> MAKMAFTLADRVTEEMLADKAALVVEVVEENYHDAPIVGIAVVNEHGRFFLRPETALADPQFVAWLGDETKKKSMFDSKRAAVALKWKGIELCGVSFDLLLAAYLLDPAQGVDDVAAAAKMKQYEAVRPDEAVYGKGAKRAVPDEPVLAEHLVRKAAAIWELERPFLDELRRNEQDRLLVELEQPLSSILAEMEFAGVKVDTKRLEQMGKELAEQLGTVEQRIYELAGQEFNINSPKQLGVILFEKLQLPVLKKTKTGYSTSADVLEKLAPYHEIVENILHYRQLGKLQSTYIEGLLKVVRPDTKKVHTIFNQALTQTGRLSSTEPNLQNIPIRLEEGRKIRQAFVPSESDWLIFAADYSQIELRVLAHIAEDDNLMEAFRRDLDIHTKTAMDIFQVSEDEVTPNMRRQAKAVNFGIVYGMSDYGLAQNLNISRKEAAEFIERYFESFPGVKRY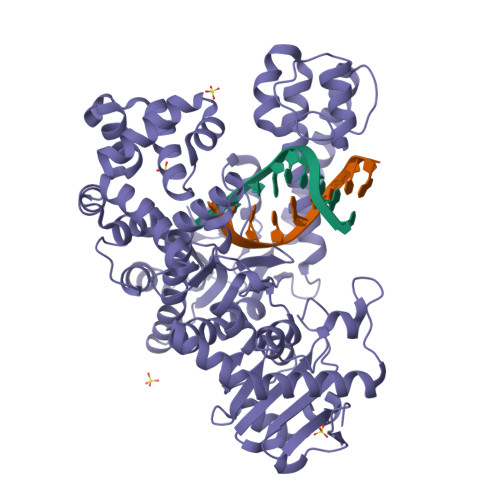MENIVQEAKQKGYVTTLLHRRRYLPDITSRNFNVRSFAERMAMNTPIQGSAADIIKKAMIDLNARLKEERLQAHLLLQVHDELILEAPKEEMERLCRLVPEVMEQAVTLRVPLKVDYHYGSTWYDAK> SMTGGQQMGRGSMDITRFKEDLKAHLEEKIIPFWQSLKDDEFGGYYGYMDFNLNIDRKAQKGCILNSRILWFFSACYNVLKSEKCKEMAFHAFEFLKNKFWDKEYEGLFWSVSHKGVPVDVTKHVYVQAFGIYGLSEYYEASGDEEALHMAKRLFEILETKCKRENGYTEQFERNWQEKENRFLSENGVIASKTMNTHLHVLESYTNLYRLLKLDDVYE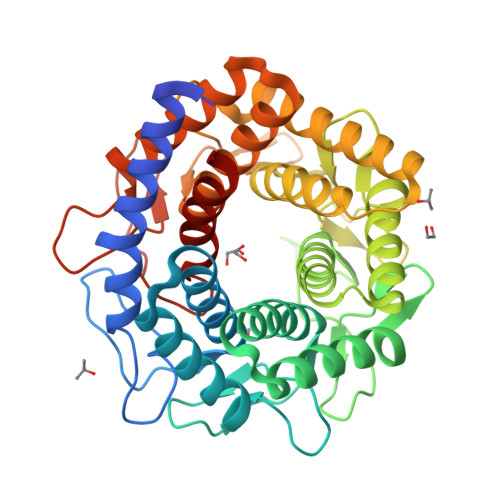ALEWIVRLFVDKIYKKGTGHFKVFCDDNWNELIKAVSYGHDIEASWLLDQAAKYLKDEKLKEEVEKLALEVAQITLKEAFDGQSLINEMIEDRIDRSKIWWVEAETVVGFFNAYQKTKEEKYLDAAIKTWEFIKEHLVDRRKNSEWLWKVNEDLEAVNMPIVEQWKCPYHNGRMCLEIIKRVD AMPylation (or adenylylation) is the transfer of AMP from ATP to a Tyr or Thr/Ser residue in target proteins. Interestingly, in eukaryotic genomes only one FIC-domain containing protein has been identified to date, HYPE or FICD, and it is strongly conserved from C. elegans to humans. Here we describe the first crystal structure of a eukaryotic HYPE encompassing the two TPR-motifs, an α-helical linker, and the FIC domain of the human protein. We demonstrate that HYPE forms stable dimers with structurally and functionally integrated FIC-domains and with TPR-motifs exposed for protein-protein interactions.

In addition to apo structures of HYPE variants, we have also obtained structures with the ATP cofactor bound to an E234G variant and with ADP bound to either the HYPE E234G variant or to wild-type protein. The position of the inhibitory glutamate (Glu234) in the structure of wild-type HYPE is consistent with its role in competing with the Arg374/γ-phospate interaction. Interestingly, there is a difference in side chain orientation of Glu234 in apo and ADP bound structures of the wild-type HYPE that shows that this side chain can also affect ADP binding and that is sufficiently flexible to accommodate bound ADP. The position of clearly visible α- and β-phosphates in all three structures is the same, with the α-phosphate present in an orientation compatible with the AMPylation reaction. Correct positioning of the α-phosphate in the wild-type HYPE/ADP complex shows that also in the case of HYPE, the γ-phosphate, and to some extent β-phosphate, could preclude efficient and/or enzymatically correct ATP binding to the wild-type protein. Wild-type HYPE also bound ADP (as the only ligand), but with a considerably lower affinity and KD of 1.5 μM, possibly owing to electrostatic repulsion by the side chain of by Glu234. Binding of ATP to wild-type HYPE could not be detected using these methods. These findings are in general agreement with the structural data and with the previously proposed role of the inhibitory Glu in obstructing correct engagement of the γ and β phosphates of ATP. Our data describing the cofactor binding, where binding of ATP to wild-type HYPE is obstructed by the conserved glutamic acid residue, raise two possibilities.

>[2x]GKLEARAALNQALEMKRQGKREKAQKLFMHALKMDPDFVDALTEFGIFSEEDKDIIQADYLYTRALTISPYHEKALVNRDRTLPLVEEIDQRYFSIIDSKVKKVMSIPKGNSALRRVMEETYYHHIYHTVAIEGNTLTLSEIRHILETRYAVPGKSLEEQNEVIGMHAAMKYINTTLVSRIGSVTISDVLEIHRRVLGYVDPVEAGRFRTTQVLVGHHIPPHPQDVEKQMQEFVQWLNSEEAMNLHPVEFAALAHYKLVYIHPFIDGNGRTSRLLMNLILMQAGYPPITIRKEQRSDYYHVLEAANEGDVRPFIRFIAKCTETTLDTLLFATTEYSVALPEAQP>[4x]MGSMAASTPVVVDIHTHMYPPSYIAMLEKRQTIPLVRTFPQA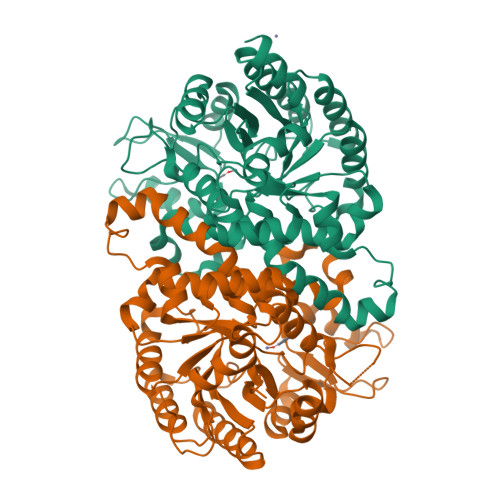DEPRLILLSSELAALDAALADPAAKLPGRPLSTHFASLAQKMHFMDTNGIRVSVISLANPWFDFLAPDEAPGIADAVNAEFSDMCAQHVGRLFFFAALPLSAPVDAVKASIERVKNLKYCRGIILGTSGLGKGLDDPHLLPVFEAVADAKLLVFLHPHYGLPNEVYGPRSEEYGHVLPLALGFPMETTIAVARMYMAGVFDHVRNLQMLLAHSGGTLPFLAGRIESCIVHDGHLVKTGKVPKDRRTIWTVLKEQIYLDAVIYSEVGLQAAIASSGADRLMFGTDHPFFPPIEEDVQGPWDSSRLNAQAVIKAVGEGSSDAAAVMGLNAVRVLSLKAELEHHHHHH(1-{[2-(3,5-dichlorophenyl)-6-{[2-(4-methylpiperazin-1-yl)pyrimidin-5-yl]oxy}pyridin-4-yl]methyl}piperidin-4-yl)acetic 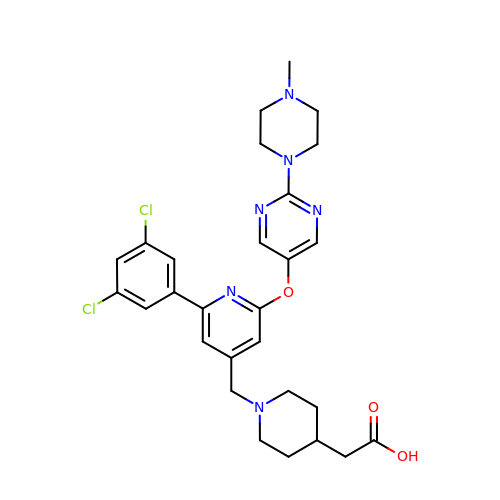acid | C28 H32 Cl2 N6 O3 | AZEJIKZNBHEXCM-UHFFFAOYSA-N>GYINVGAQLGTELFIVRQLLQIVKQKTNQNSVDTTLKFTLSALWNLTDESPTTCRHFIENQGLELFMRVLESFPTESSIQQKVLGLLNNIAEVQELHSELMWKDFIDHISSLLHSVEVEVSYFAAGIIAHLISRGEQAWTLSRSQRNSLLDDLHSAILKWPTPECEMVAYRSFNPFFPLLGCFTTPGVQLWAVWAMQHVCSKNPS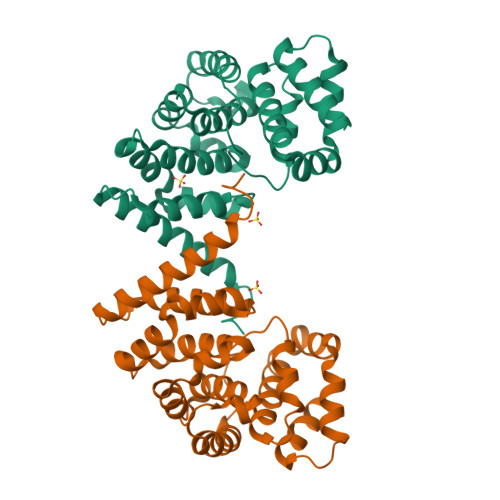RYCSMLIEEGGLQHLYNIKDHEHTDPHVQQIAVAILDSLEKHIVR[2x]>MTLEAIRYSRGSLQILDQLLLPKQSRYEAVGSVHQAWEAIRAMKVRGAPAIALVGCLSLAVELQAGAGGPGLAALVAFVRDKLSFLVTARPTAVNMARAARDLADVAAREAEREGATEEAVRERVICCTEDMLEKDLRDNRSIGDLGARHLLERVAPSGGKVTVLTHCNTGALATAGYGTALGVIRSLHSLGRLEHAFCTETRPYNQGARLTAFELVYEQIPATLITDSMVAAAMAHRGVSAVVVGADRVVANGDTANKVGTY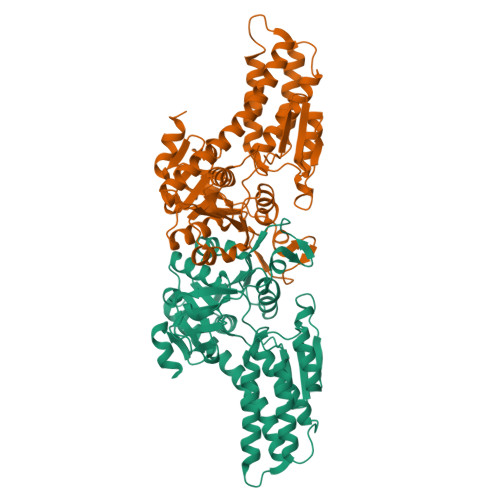QLAIVAKHHGIPFYVAAPSYSCDLRLETGKEIIIEERPGQELTDVNGVRIAAPGIGVWNPAFDVTPHDLITGGIITELGVFAPEELRTALTTTISSRDGTLDGPQM[2x]> MGRDPNSDQTAEIVIHKRIYRDIRQPEDVWYENDGHRIDPNNPDKDGYKLLSKTSGLNGANFEVYDASSLLKPNMTPEAIRALVDRYQNMTRKQALKFARANLKLAGQGNKGIGLMNTKNDPTLGEDGISRITVSVDQQAPTKAYLMIEVAPDPSTELNVDLERKSSPMLVVFPVTDPISGNPLQTIHLYPKNVGYVRDPYFFKFGVHPDGTSKRLAGAIFAIYRIENGKKLYLDMSPVTDLRNKWVSTTDPLHDDRVNKFVSDQDGLVNTGER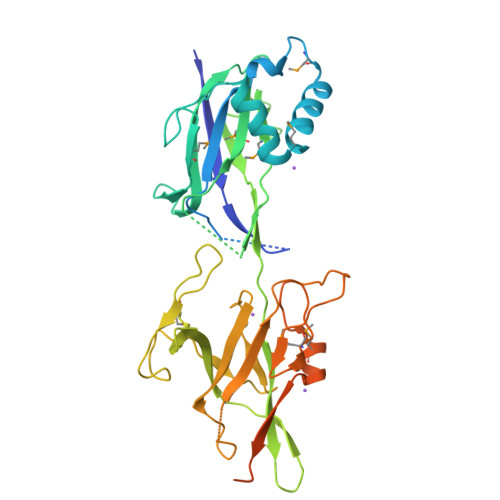FLPAGEYFFEELQGVPGYEVDAKSRAIKIEIPDSWEDEDGNRRFVLIDGQPMQENFGGVVTPEMISSGYPRVYNYADKQASTTGDQTAGPSTTQLGNHGQDTNGTGTRTPKRQSGYLPLEHHHHHH> MGSSHHHHHHSSGLVPRGSHMMNTFSSFRKHALLHSKETAVKSINHNISFYNLLLLIQRIATGLKSANIKKGDRISIHMGNCFELIATYYACLKIGAVFVPLSLKLSAKEVKNLIQHSSSCAYIGDKKRFYETKQEIESCTMLEKIWVIDLKIEDKENNTHNWEEIISQPYDYSEDNIYTDEIASIFYTSGTTGHPKGIVYSQKTLIDAVNLTKVTINPRLPKSDGDKPAILSLVDLISPWSILITFAALQKGYSVLLLSEVDIENITETLKETQPAWIAGTPSNFHKIIKNEENNNNSLDLSETVCVAGGDSCATELSQKFFECFGSHLQSSYGQTELGGPVIYHHDIYAINEPSIGWPLPGVEIKINNTQSSNGELLIRSPAKTIGIWNGH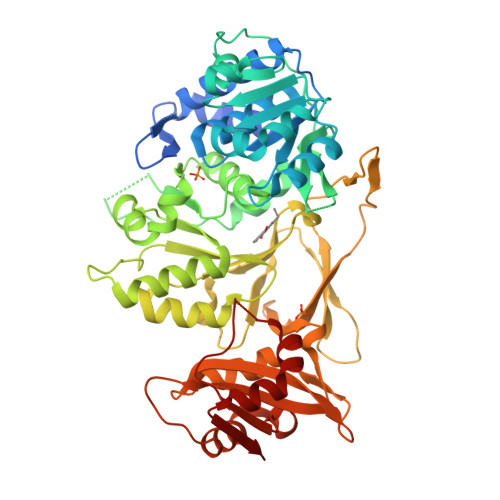DIELFPSDRWLATGDLVRQENNGNLIFLGREKDQIKIEGYPVYPIEIENTLIQHADIAASVVFSVPDKYAGERIIALIQPQKNHSLKAETIASYLSDNLAHYKHPSEYIFIKEIPVNTTGKISRRKLSNEYHLLKSQAEKVFTL>GPGSKPFTLPILTLGELTNSRFPLPIDVLYTNPNESAIVQCQNGRCTLDGELQGTTQLLPTGICAFRGKV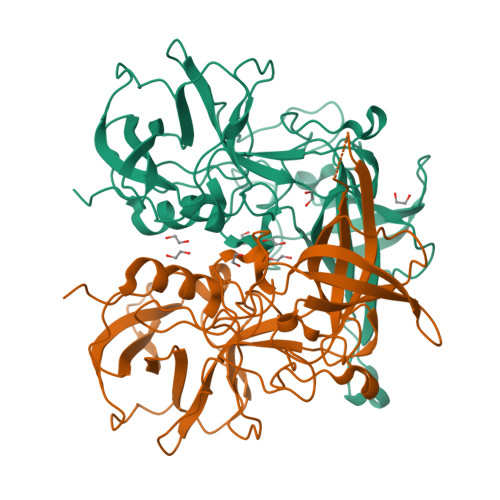TQQVQDEHRGTHWNMTVTNLNGTPFDPTEDVPAPLGTPDFSGQIYGVISQRNTNTVPGEGNLPANRAHEAVIATYSPKFTPKLGNIQFSTWETQDVSSGQPTKFTPVGLASVDANSHFDQWTLPSYSGALTLNMNLAPSVAPVFPGECLLFFRSFIPLKGGYGNPAIDCLMPQEWVQHLYQESAPSLSDVALVRYVNPETGRTLFEAKLHRNGFLTVARNSAGPVVAPTNGYFRFDSWVNQFYTLAPM[2x]> GSHMASPNGQTKPLPALKLALEYIVPCMNKHGICVVDDFLGKETGQQIGDEVRALHDTGKFTDGQLVSQKSDSSKDIRGDKITWIEGKEPGCETIGLLMSSMDDLIRHCNGKLGSYKINERTKAMVACYPGNGTGYVRHVDNPNGDGRCVTCIYYLNKDWDAKVSGGILRIFPEGKAQFADIEPKFDRLLFFWSDRRNPHEVQPAYATRYAITVWYFDADERARAKVKYLTGEKGVRVELNKPSDSVGKDVF

The ferrous iron and 2-oxoglutarate (2OG)-dependent HIF prolyl hydroxylases (PHDs/EGLNs) catalyse trans-4-prolyl hydroxylations on HIFα subunits, thus promoting their binding to the von Hippel–Lindau protein (VHL), a targeting component of a ubiquitin E3 ligase, and signalling for HIFα degradation under normoxic conditions. The PHD-catalysed hydroxylations of HIF-1α/HIF-2α in higher animals occur in amino- and carboxy-terminal oxygen-dependent degradation domains (NODD and CODD). The three human PHDs exhibit different NODD/CODD selectivities, with PHD3 being substantially more selective for CODD than PHD1/2 (refs 16). Biophysical analyses employing crystallography and NMR reveal that the molecular basis of PHD isoform and variant selectivity involves enzyme–substrate interactions involving β2/β3 loop residues (that bind the LXXLAP motif) and helices α3 and α4, regions which display sequence variations between the PHD isoforms.

Using biochemical and structural studies, we identified four more residues in α3 and α3-βI loop regions (PHD2/Ile280, Arg281, Ile292 and Gly294 that are substituted in PHD3/Val102, Leu103, Val114 and Glu116, respectively) and which play roles in determining selectivity. Indeed, we found that FG2216 (IOX3)35, used in clinical trials for treatment of anaemia, preferentially displaces NODD over CODD from PHD2.(1R,3R)-3-(2-methylimidazo[4,5-d]pyrrolo[2,3-b]pyridin-1(8H)-yl)cyclohexanol | C15 H18 N4 O | 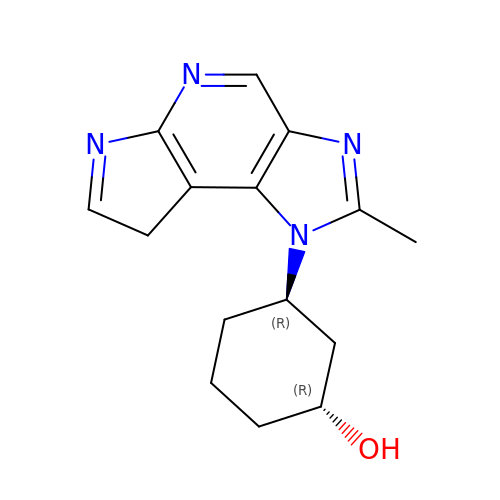IWJKSSOUXRKEPE-GHMZBOCLSA-N>HHHHHHMLENIRDAVRKFLTGSTPYEKAVDEFIKDLQKSLISSDVNVKLVFSLTAKIKERLNKEKPPSVLERKEWFISIVYDELSKLFGGDKEPNVNPTKLPFIIMLVGVQGSGKTTTAGKLAYFYKKRGYKVGLVAADVYRPAAYDQLLQLGNQIGVQVYGEPNNQNPIEIAKKGVDIFVKNKMDIIIVDTAGRHGYGEETKLLEEMKEMYDVLKPDDVILVIDASIGQKAYDLASRFHQASPIGSVIITKMDGTAKGGGALSAVVATGATIKFIGTGEKIDELETFNAKRFVSRIL[4x];>[4x]HHHHHHRSFFDFLKYKTIKEDDLNDVIEELRFQLLDSDVSYE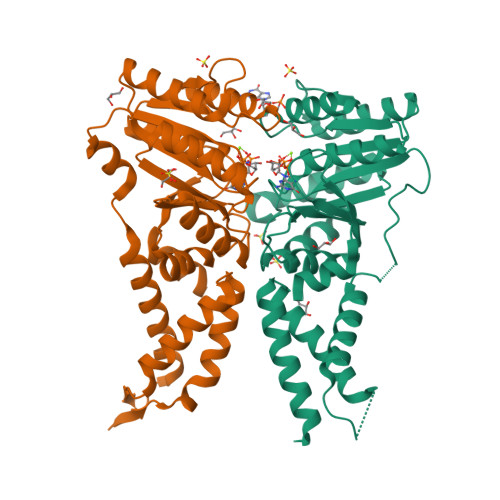VTEKILEDLKNNLIGKKVSRREEVEEIVINTLKKSITEILTKNQKTDLIEKIRSSGKKPFVIIFFGVNGVGKTTTIAKVVNMLKKNNLSTIIAASDTFRAAAQEQLAYHASKLEVQLIRGKYGADPASVAFDAISFAKSRNIDVVLIDTAGRMHIDSDLVEELKKVLRIAKPDFRILILDSLAGSDALEQARHFENNVGYDAVILTKVDADAKGGIALSLAYELKKPVVYMGVGQNYDDLIPFSPDWFVERIFS>GAVELLVFNFLLILTILTIWLFKNHRFRFLHETGGAMVYGLIMGLILRYATAPTDIESGTVYDCGKLAFSPSTLLINITDQVYEYKYKREISQHNINPHLGNAILEKMTFDPEIFFNVLLPPIIFHAGYSLKKRHFFQNLGSILTYAFLGTAISCIVIGLIMYGFVKAMVYAGQLKNGDFHFTDCLFFGSLMSATDPVTVLAIFHELHVDPDLYTLLFGESVLNDAVAIVLTYSISIYSPKENPNAFDAAAFFQSVGNFLGIFAGSFAMGSAYAVVTALLTKFTKLCEFPMLETGLFFLLSWSAFLSAEAAGLTGIVAVLFCGVTQAHYTYNNLSLDSKMRTKQLFEFMNFLAENVIFCYMGLA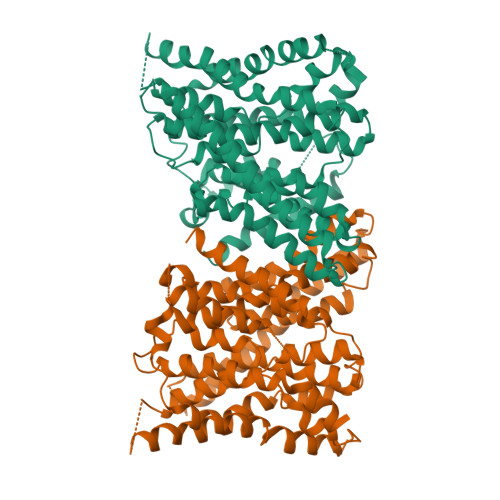LFTFQNHIFNALFILGAFLAIFVARACNIYPLSFLLNLGRKHKIPWNFQHMMMFSGLRGAIAFALAIRDTESQPKQMMFSTTLLLVFFTVWVFGGGTTGENLYFQ[2x]(1S)-4-fluoro-1-(4-fluoro-3-pyrimidin-5-ylphenyl)-1-[2-(trifluoromethyl)pyridin-4-yl]-1H-isoindol-3-amine 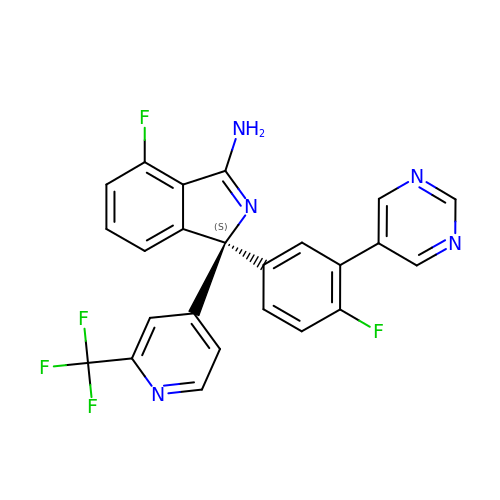| C24 H14 F5 N5 | UDQUVXUVXUGJFO-QHCPKHFHSA-N>[2x]LVSSPTSSGLYVVHIAAEMAPVAKVGGLGDVVAGLGKALQRKGHLVEIILPKYDCMQYDRVRDLRALDTVVESYFDGKLYKNKIWIGTVEGLPVHFIEPQHPSKFFWRGQFYGEQDDFRRFSYFSRAALELLLQSGKKPDIIHCHDWQTAFVAPLYWDLYAPKGLDSARICFTCHNFEYQGTASASELGSCGLDVNQLNRPDRMQDHSSGDRVNPVKGAIIFSNIVTTVSPTYAQEVRTAEGGKGLHSTLNFHSKKFIGILNGIDTDSWNPATDPFLKAQFNAKDLQGKEENKHALRKQLGLSSAESRRPLVGCITRLVPQKGVHLIRHAIYRTLELGGQFVLLGSSPVPHIQREFEGIEQQFKSHDHVRLLLKYDEALSHTIYAASDLFIIPSIFEPCGLTQMIAMRYGS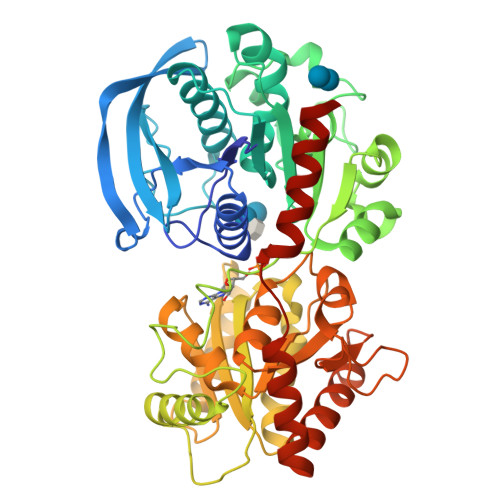IPIARKTGGLNDSVFDIDDDTIPTQFQNGFTFQTADEQGFNYALERAFNHYKKDEEKWMRLVEKVMSIDFSWGSSATQYEELYTRSVSRARAVPNRT>MRSRRVDVMDVMNRLILAMDLMNRDDALRVTGEVREYIDTVKIGYPLVLSEGMDIIAEFRKRFGCRIIADFKVADIPETNEKICRATFKAGADAIIVHGFPGADSVRACLNVAEEMGREVFLNTEMSHPGAEMFIQGAADEIARMGVDLGVKNYVGPSTRPERLSRLREIIGQDSFLISPGVGAQGGD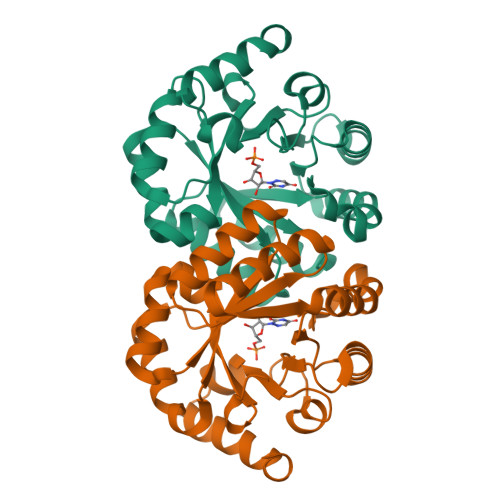PGETLRFADAIIVGRSIYLADNPAAAAAGIIESIKDLLNP[2x]> DMPRPTGLAADIRWTAYGVPHIRAKDERGLGYGIGYAYARDNACLLAEEIVTARGERARYFGSEGKSSAELDNLPSDIFYAWLNQPEALQAFWQAQTPAVRQLLEGYAAGFNRFLREADGKTTSCLGQPWLRAIATDDLLRLTRRLLVEGGVGQFADALVAAAPPGAEKV;> SNAIAVGSERSADGKGMLLANPHFPWNGAMRFYQMHLTIPGRLDVMGASLPGLPVVNIGFSRHLAWTHTVDTSSHFTLYRLALDPKDPRRYLVDGRSLPLEEKSVAIEVRGADGKLSRVEHKVYQSIYGPLVVWPGKLDWNRSEAYALRDANLENTRVLQQWYSINQASDVADLRRRVEALQGIPWVNTLAADEQGNALYMNQSVVPYLKPELIPACAIPQLVAEGLPALQGQDSRCAWSRDPAAAQAGITPAAQLPVLLRRDFVQNSNDSAWLTNPASPLQGFSPLVSQEKPIGPRARYALSRLQGKQPLEAKTLEEMVTANHVFSADQVLPDLLRLCRDNQGEKSLARACAALAQWDRGANLDSGSGFVYFQRFMQRFAELDGAWKEPFDAQRPLDTPQGIALDRPQVATQVRQALADAAAEVEKSGIPDGARWGDLQVSTRGQERIAIPGGDGHF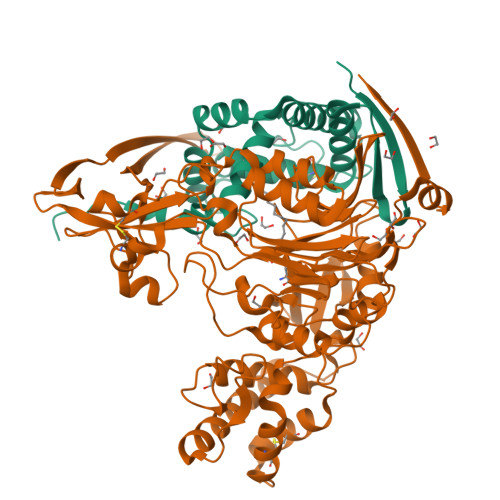GVYNAIQSVRKGDHLEVVGGTSYIQLVTFPEEGPKARGLLAFSQSSDPRSPHYRDQTELFSRQQWQTLPFSDRQIDADPQLQRLSIRE>CFLHVGAQLGTELFIVRQLLQIVKQKTNQNSVDTTLKFTLSALWNLTDESPTTCRHFIENQGLELFMRVLESFPTESSIQQKVLGLLNNIAEVQELHSELMWKDFIDHISSLLHSVEVEVSYFAAGIIAHLISRGEQAWTLSRSQRNSLLDDLHSAILKWPTPECEMVAYRSFNPFFPLLGCFTTPGVQLWAVWAMQHVCSKNPSRYCSML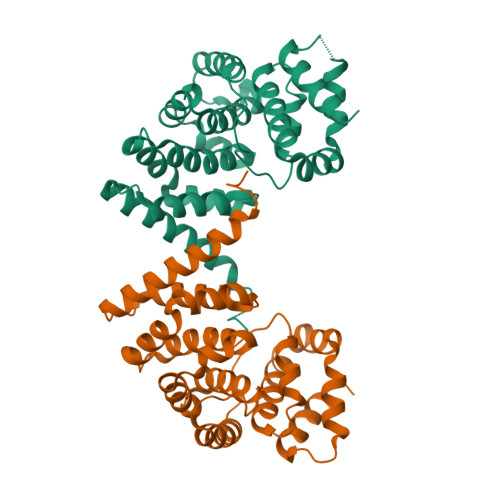IEEGGLQHLYNIKDHEHTDPHVQQIAVAILDSLEKHIVR[2x]> MEFDDDLVDAEGNLVEDGGTYYLLPHIWAHGGGIETAKTGNEPCPLTVVRSPNEVSKGEPIRISS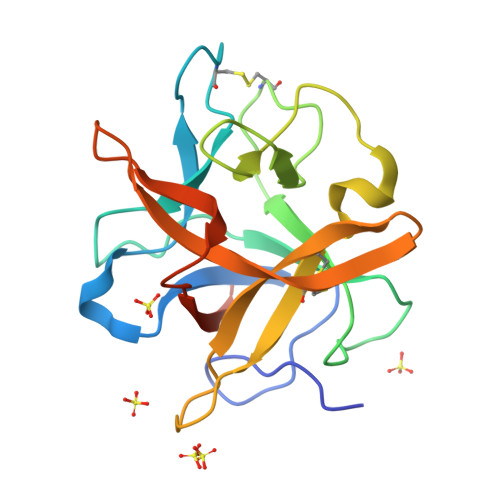QFLSLFIPRGSLVALGFANPPSCAASPWWTVVDSPQGPAVKLSQQKLPEKDILVFKFEKVSHSNIHVYKLLYCQHDEEDVKCDQYIGIHRDRNGNRRLVVTEENPLELVLLKAKSETASSH>MEEAKQKVVDFLNSKSGSKSKFYFNDFTDLFPDMKQREVKKILTALVNDEVLEYWSSGSTTMYGLKGA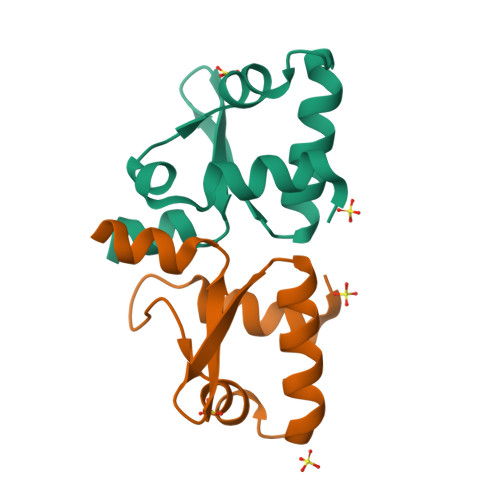GKQAAAEHED[2x]>AELPPGRLATTEDYFAQQAKQAVTPDVMAQLAYMNYIDFISPFYSRGCSFEAWELKHTPQRVIKYSIAFYAYGLASVALIDPKLRALAGHDLDIAVSKMKCKRVWGDWEEDGFGTDPIEKENIMYKGHLNLMYGLYQLVTGSRRYEAEHAHLTRIIHDEIAANPFAGIVCEPDNYFVQCNSVAYLSLWVYDRLHGTDYRAATRAWLDFIQKDLIDPERGAFYLSYHPESGAVKPWISAYTTAWTLAMVHGMDPAFSERYYPRFKQTFVEVYDEGRKARVRETAGTDDADGGVGLASAFTL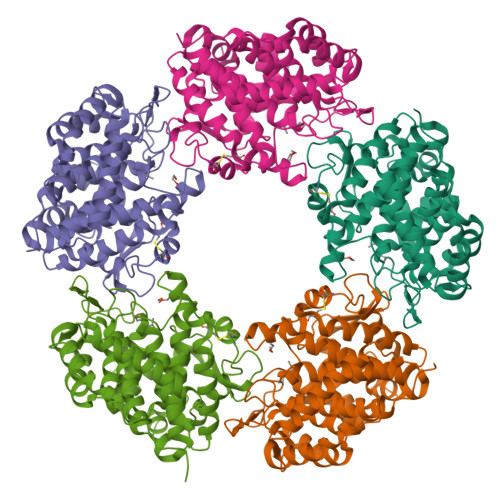LLAREMGDQQLFDQLLNHLEPPAKPSIVSASLRYEHPGSLLFDELLFLAKVHAGFGALLRMPPPAAKLAGK[5x]> GSKVEDPKDFPSELLSFLSHAVCSNRTLACFAIYTTKEKAALLYKKIMEKYSVTFISRHNSYNHN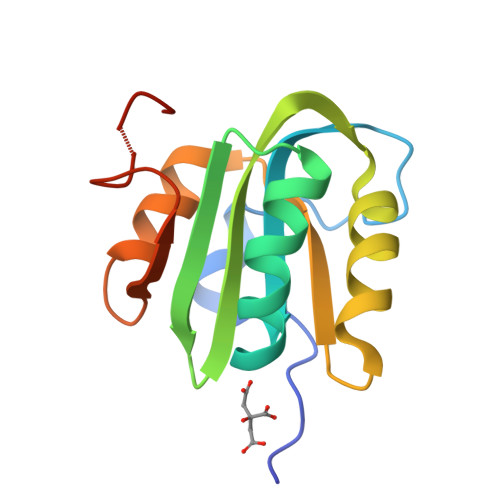ILFFLTPHRHRVSAINNYAQKLATFSFLICKGVNKEYLMYSALTRDPFSVIEESLPGGLKEHCFNPESS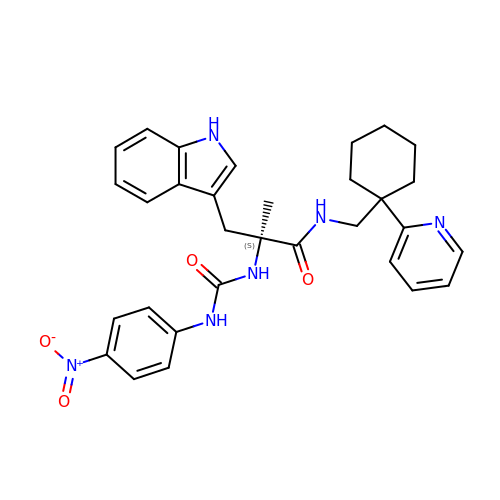(2~{S})-3-(1~{H}-indol-3-yl)-2-methyl-2-[(4-nitrophenyl)carbamoylamino]-~{N}-[(1-pyridin-2-ylcyclohexyl)methyl]propanamide | C31 H34 N6 O4 | AFDXUTWMFMAQJO-PMERELPUSA-N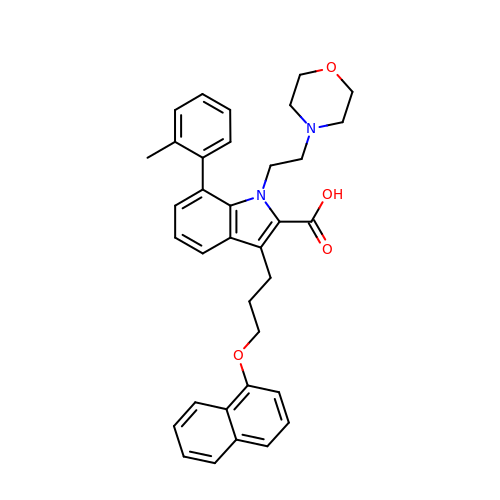7-(2-methylphenyl)-1-[2-(morpholin-4-yl)ethyl]-3-{3-[(naphthalen-1-yl)oxy]propyl}-1H-indole-2-carboxylic acid | C35 H36 N2 O4 | ZFODCXXHTZVRJL-UHFFFAOYSA-N> EFMETYVNKLHEGSTYTAAVQY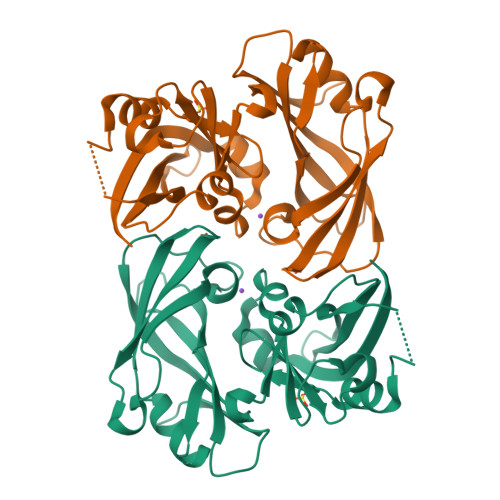NVLEKDDDPASLTIWVPMFQSSMPADLLIKELANVNILVKQISTPKGPSLRVMINSRSAVLAQMPSKFTICANVSLDERSKLAYDVTTPCEIKACSLTCLKSKNMLTTVKDLTMKTLNPTHDIIALCEFENIVTSKKVIIPTYLRSISVRNKDLNTLENITTTEFKNAITNAKIIPYSGLLLVITVTDNKGAFKYIKPQSQFIVDLGAYLEKESIYYVTTNWKHTATRFAIKPMED N-methylquinolin-2-amine 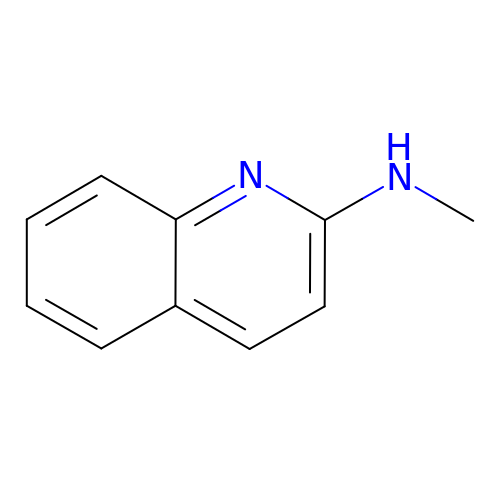| C10 H10 N2 | POVSMFKXVSNGSU-UHFFFAOYSA-N> MLSVLRPFPSPLLSRHGIDLDFPLLAGCLALLGLGLVMVTSASSEVAAAQSGNPLYFSVRHLIYLVIGLISCGLTMMVPMATWQRWGWKLLLVAFGLLVLVITPGIGREVNGSMRWIGFGLFNIQPSEIAKVCVVIFMAGYLIRRQQEVRESWMGFFKPFVVLLPMAGLLLREPDFGATVVMMGAAAAMLFLGGVGLFRFGLMVLLAVGAVVLLIQTQPYRMARLTNFTDPWADQFGAGYQLSQALIAFGRGGWLGMGLGNSIQKQFYLPEAHTDFVFAVLAEELGIVGALATVALFVFVSLRALYIGIWAEQAKQFFSAYVAYGLAFLWIGQFLINIGVNVGLLPTKGLTLPFLSYGGSSLVICCACLGMLLRIEWERRTHLGSEEYEFNEEDFADER;> MKLNYFQGALYPWRFCVIVGLLLAMVGAIVWRIVDLHVIDHDFLKGQGDARSVRHIAIPAHRGLITDRNGEPLAVSTPVTTLWANPKELMTAKERWPQLAAALGQDTKLFADRIEQNAEREFIYLVRGLTPEQGEGVIALKVPGVYSIEEFRRFYPAGEVVAHAVGFTDVDDRGREGIELAFDEWLAGVPGKRQVLKDRRGRVIKDVQVTKNAKPGKTLALSIDLRLQYLAHRELRNALLENGAKAGSLVIMDVKTGEILAMTNQPTYNPNNRRNLQPAAMRNRAMIDVFEPGSTVKPFSMSAALASGRWKPSDIVDVYPGTLQIGRYTIRDVSRNSRQLDLTGILIKSSNVGISKIAFDIGAESIYSVMQQVGLGQDTGLGFPGERVGNLPNHRKWPKAETATLAYGYGLSVTAIQLAHAYAALANDGKSVPLSMTRVDRVPDGVQVISPEVASTVQGMLQQVVEAQGGVFRAQVPGYHAAGKSGTARKVSVGTKGYRENAYRSLFAGFAPATDPRIAMVVVIDEPSKAGYFGGLVSAPVFSKVMAGALRLMNVPPDNLPTATEQQQVNAAPAKGGRG;> MSRLFVKRLPTGSFLMLLLYIGLLLSAIAVAYSTYWNRQLLNSLYSELSVRDKAQAEWGRLILEQSTWTAHSRIESLAVEQLRMRVPDPAEVRMVAP;> MRLRSPYWLFVVLILALAGLQY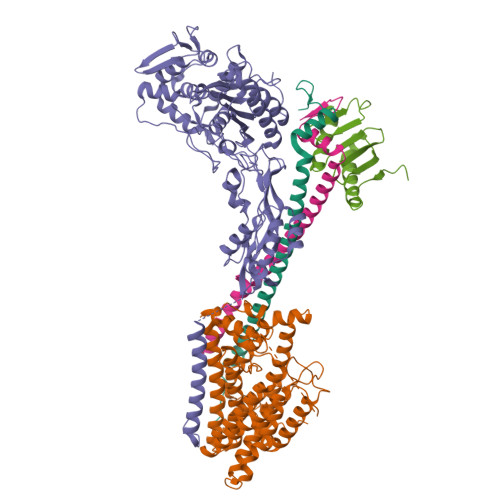RLWVGDGSLAQVRDLQKQIADQHGENERLLERNRILEAEVAELKKGTETVEERARHELGMVKDGETLYQLAK;> MNGVLLRHQQPGGLGRAPRKPMPRGASRLVAKEPLSVRLPKADFSFLKYLAWPLLLAVLGYGAYRGAEYILPYADRPIAKVSVEGDLSYISQRAVQQRISPYLAASFFTIDLAGMRGQLEQMPWIAHAEVRRVWPDQVVIRLDEQLPIARWGDEALLNNQGQAFTPKELANYEHLPRLHGPQRAQQQVMQQYQLLSQLLRPLGFSIARLEMSDRGGWALTTAQGVEIQIGRDHVVDKIRRFVSIYDKALKDQISNIARIDLRYPNGLAVAWREPVTPATVATASAVQ>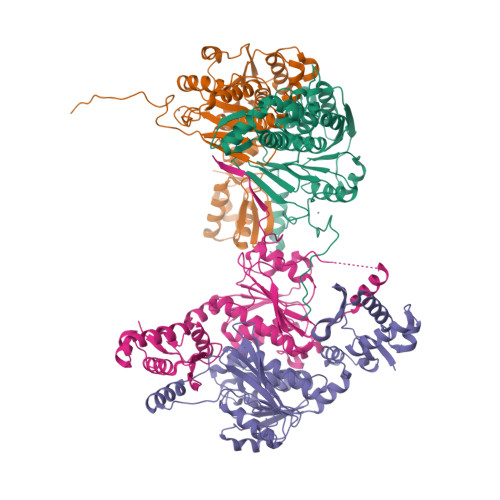MDYILGRYVKIARYGSGGLVGGGGKEQYVENLVLWENIIKTAYCFITPSSYTAALETANIPEKDFSNCFRFLKENFFIIPGEYNNSTENNRYSRNFLHYQSYGANPVLVQDKLKNAKVVILGCGGIGNHVSVILATSGIGEIILIDNDQIENTNLTRQVLFSEDDVGKNKTEVIKRELLKRNSEISVSEIALNINDYTDLHKVPEADIWVVSADHPFNLINWVNKYCVRANQPYINAGYVNDIAVFGPLYVPGKTGCYECQKVVADLYGSEKENIDHKIKLINSRFKPATFAPVNNVAAALCAADVIKFIGKYSEPLSLNKRIGIWSDEIKIHSQNMGRSPVCSVCGNRMLEHHHHHH[4x]>[3x]ELVKGVYAKYWIYVCAGMFIVVSFAGRLVVYKIVYMFLFLLCLTLFQVYYSLWRKLLKAFWWLVVAYTMLVLIAVYTFQFQDFPAYWRNLTGFTDEQLGDLGLEQFSVSELFSSILVPGFFLLACILQLHYFHRPFMQLTDMEHVSLPGTRLPRWAHRQDAVSGTPLLREEQQEHQQQQQEEEEEEEDSRDEGLGVATPHQATQVPEGAAKWGLVAERLLELAAGFSDVLSRVQVFLRRLLELHVFKLVALYTVWVALKEVSVMNLLLVVLWAFALPYPRFRPMASCLSTVWTCVIIVCKMLYQLKVVNPQEYSSNCTEPFPNSTNLLPTEISQSLLYRGPVDPANWFGVRKGFPNLGYIQNHLQVLLLLVFEAIVYRRQEHYRRQHQLAPLPAQAVFASGTRQQLDQDLLGCLKYFINFFFYKFGLEICFLMAVNVIGQRMNFLVTLHGCWLVAILTRRHRQAIARLWPNYCLFLALFLLYQYLLCLGMPPALCIDYPWRWSRAVPMNSALIKWLYLPDFFRAPNSTNLISDFLLLLCASQQWQVFSAERTEEWQRMAGVNTDRLEPLRGEPNPVPNFIHCRSYLDMLKVAVFRYLFWLVLVVVFVTGATRISIFGLGYLLACFYLLLFGTALLQRDTRARLVLWDCLILYNVTVIISKNMLSLLACVFVEQMQTGFCWVIQLFSLVCTVKGYYDPKEMMDRDQDCLLPVEEAGIIWDSVCFFFLLLQRRVFLSHYYLHVRADLQATALLASRGFALYNAANLKSIDFHRRIEEKSLAQLKRQMERIRAKQEKHRQGRVDRSRPQDTLGPKDPGLEPGPDSPGGSSPPRRQWWRPWLDHATVIHSGDYFLFESDSEEEEEAVPEDPRPSAQSAFQLAYQAWVTNAQAVLRRRQQEQEQARQEQAGQLPTGGGPSQEVEPAEGPEEA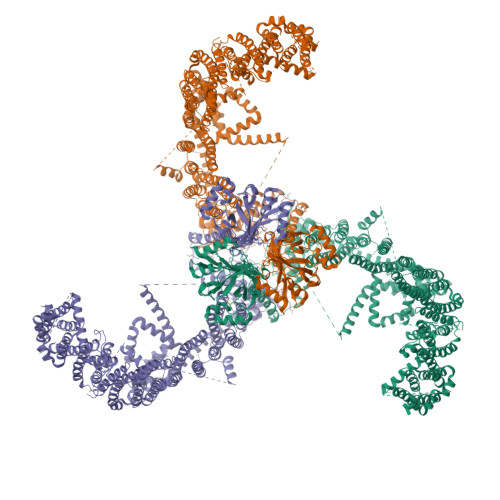AAGRSHVVQRVLSTAQFLWMLGQALVDELTRWLQEFTRHHGTMSDVLRAERYLLTQELLQGGEVHRGVLDQLYTSQAEATLPGPTEAPNAPSTVSSGLGAEEPLSSMTDDMGSPLSTGYHTRSGSEEAVTDPGEREAGASLYQGLMRTASELLLDRRLRIPELEEAELFAEGQGRALRLLRAVYQCVAAHSELLCYFIIILNHMVTASAGSLVLPVLVFLWAMLSIPRPSKRFWMTAIVFTEIAVVVKYLFQFGFFPWNSHVVLRRYENKPYFPPRILGLEKTDGYIKYDLVQLMALFFHRSQLLCYGLWDHEEDSPSKEHDKSGEEEQGAEEGPGVPAATTEDHIQVEARVGPTDGTPEPQVELRPRDTRRISLRFRRRKKEGPARKGAAAIEAEDREEEEGEEEKEAPTGREKRPSRSGGRVRAAGRRLQGFCLSLAQGTYRPLRRFFHDILHTKYRAATDVYALMFLADVVDFIIIIFGFWAFGKHSAVTDITSSLSDDQVPEAFLVMLLIQFSTMVVDRALYLRKTVLGKLAFQVALVLAIHLWMFFILPAVTERMFNQNVVAQLWYFVKCIYFALSAYQIRCGYPTRILGNFLTKKYNHLNLFLFQGFRLVPFLVELRAVMDWVWTDTTLSLSSWMCVEDIYANIFIIKCSRETEKKYPQPKGQKKKKIVKYGMGGLIILFLIAIIWFPLLFMSLVRSVVGVVNQPIDVTVTLKLGGYEPLFTMSAQQPSIIPFTAQAYEELSRQFDPQPLAMQFISQYSPEDIVTAQIEGSSGALWRISPPSRAQMKRELYNGTADITLRFTWNFQRDLAKGGTVEYANEKHMLALAPNSTARRQLASLLEGTSDQSVVIPNLFPKYIRAPNGPEANPVKQLQPNEEADYLGVRIQLRREQGAGATGFLEWWVIELQECRTDCNLLPMVIFSDKVSPPSLGFLAGYGIMGLYVSIVLVIGKFVRGFFSEISHSIMFEELPCVDRILKLCQDIFLVRETRELELEEELYAKLIFLYRSPETMIKWTREKE> ETPPRFTRTPVDQTGVSGGVASFICQATGDPRPKIVWNKKGKKVSNQRFEVIEFDDGSGSVLRIQPLRTPRDEAIYECVASNNVGEISVSTRLTVLREDQIPRGFPTIDMGPQLKVV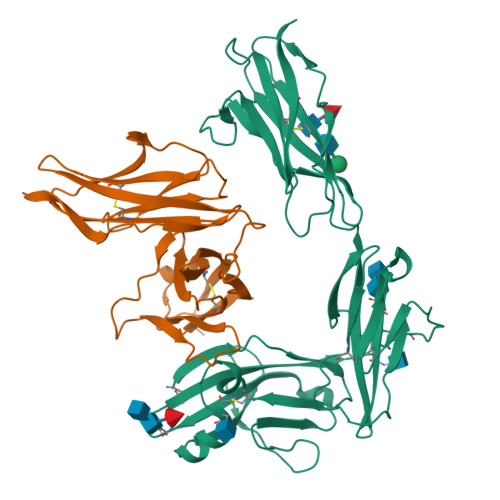ERTRTATMLCAASGNPDPEITWFKDFLPVDTSNNNGRIKQLRSESIGGTPIRGALQIEQSEESDQGKYECVATNSAGTRYSAPANLYVRELREVRRVPPRFSIPPTNHEIMPGGSVNITCVAVGSPMPYVKWMLGAEDLTPEDDMPIGRNVLELNDVRQSANYTCVAMSTLGVIEAIAQITKHHHHHH;> PAARDLKVVTKRGSADGCTDWSVDIKKYQVLVGEPVRIKCALFYGYIRTNYSLAQSAGLSLMWYKSSGPGDFEEPIAFDGSRMSKEEDSIWFRPTLLQDSGLYACVIRNSTYCMKVSISLTVGENDTGLCYNSKMKYFEKAELSKSKEISCRDIEDFLLPTREPEILWYKECRTKAWRPSIVFKRDTLLIKEVKEDDIGNYTCELKYGGFVVRRTTELTVTAPLTDKPPKLLYPMESKLTVQETQLGGSANLTCRAFFGYSGDVSPLIYWMKGEKFIEDLDENRVWESDIRILKEHLGEQEVSISLIVDSVEEGDLGNYSCYVENGNGRRHASVLLHKRKHHHHHH> MVANPEHYIKHPLQNRWALWFFKNDKSKTWQANLRLISKFDTVEDFWALYNHIQLSSNLMPGCDYSLFKDGIEPMWEDEKNKRGGRWLITLNKQ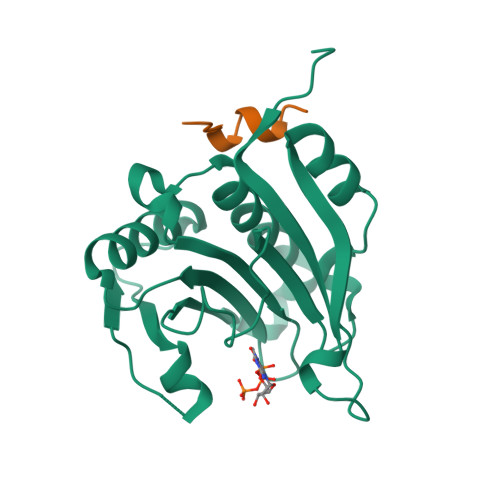QRRSDLDRFWLETLLCLIGESFDDYSDDVCGAVVNVRAKGDKIAIWTTECENREAVTHIGRVYKERLGLPPKIVIGYQSHADTATKSGSTTKNRFVV>PVSVDGETLTVEAVRRVAEERATVDVPAESIAKAQKSREIFEGIAEQNIPIYGVTTGYGEMIYMQVDKSKEVELQTNLVRSHSAGVGPLFAEDEARAIVAARLNTLAKGHSAVRPIILERLAQYLNEGITPAIPEIGSLGASGDLAPLSHVASTLIGEGYVLRDGRPVETAQVLAERGIEPLELRFKEGLALINGTSGMTGLGSLVVGRALEQAQQAEIVTALLIEAVRGSTSPFLAEGHDIARPHEGQIDTAANMRALMRGSGLTVEHADLRRELQKDKEAGKDVQRSEIYLQKAYSLRAIPQVVGAVRDTLYHARHKLRIELNSANDNPLFFEGKEIFHGANFHGQPIAFAMDFVTIALTQLGVLAERQINRVLNRHLSYGLPEFLVSGDPGLHSGFAGAQYPATALVAENRTIGPASTQSVPSNGDNQDVVSMGLISARNA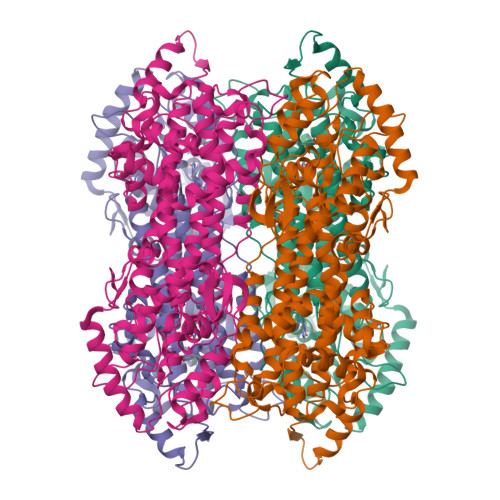RRVLSNNNKILAVEYLAAAQAVDISGRFDGLSPAAKATYEAVRRLVPTLGVDRYMADDIELVADALSRGEFLRAIARETDIQLR[2x]>GSHMTADK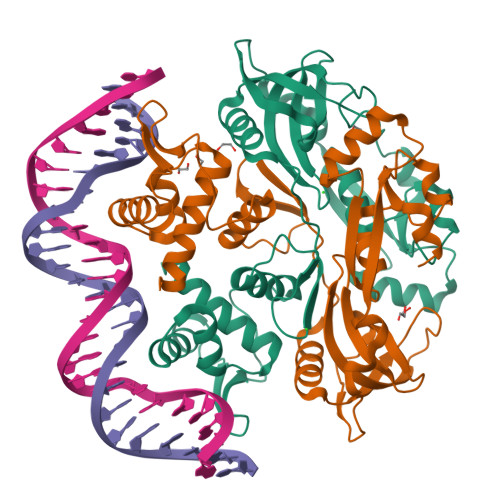HEVLLRMRAIELLAYWEGRLVTTRLMNWFGLSRQQASADIKRYNTLYNPDALIHDPSVKGYVPKASFQPVLTTAHINEYLNMLSGLVSESHALIAMPEPNLAAVQLPDRSVRPEVIREVLRACRNQSTLKMIYASMQNPQWHERIISPHTLVYTGFRWHVRAYCHQSKQFKDFLLSRIDRTPVVVAIESVDPAQDQQWHEEIVLTLIPNPKLNSSQQALVEKDFGMPDGRLQIPVKKALAHYTLQRYQTAITLAEAEDALKYPLVLQRSDIEKLSSYLFDQAS[2x]>SNAMKQTVYTASPESQQIHVWSLEADGKLTLVQVVDAPGQVQPMVVSPNKEFLYVGVRPEFRVLAYRITPDNGALTFAGEAALPGSPTHISTDRHGRFVFSASYNQGCVSVTPLHDGLPGETITVVEGLEGCHSANISPDNRTLWVPALKQDRICLFTLSDDGFLSAQEPAEVTTVEGAGPRHMVFHPNQQYGYCVNELNSSIDVWELKDPKGNIECVQTLDMMPPDFSGVRWAADIHITPDGRHLYACDRTASIITVFSVSEDGSVLAVEGYQPTETQPRGFNLDHSGKYLIAA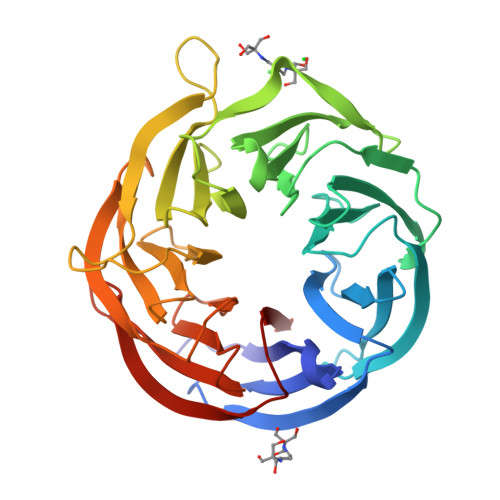GQKSHHIAVYDIVGEQGLLQEKGRYAVGQGPMWVVVNAH[3x]> PLGSEEEEEDAGLVAEAEAVAAGWMLDFLCLSLCRAFRDGRSEDFRRTRNSAEAIIHGLSSLTACQLRTIYICQFLTRIAAGKTLDAQFENDERITPLESALMIWGSIEKEHDKLHEEIQNLIKIQAIAVCMENGNFKEAEEVFERIFGDPNSHMPFKSKLLMIISQKDTFHSFFQHFSYNHMMEKIKSYVNYVLSEKSSTFLMKAAAKVVESKR;> SGAVTSFLHSLIIQNEPRFAMFGPGLEELNTSLVLSLMSSEELCPTAGLPQRQIDGIGSGVNFQLNNQHKFNILILYSTTRKERDRAREEHTSAVNKMFSRHNEGDDQQGSRYSVIPQIQKVCEVVDGFI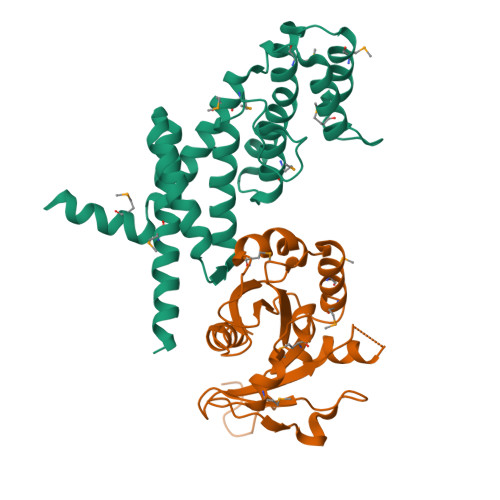YVANAEAHKRHEWQDEFSHIMAMTDPAFGSSGRPLLVLSCISQGDVKRMPCFYLAHELHLNLLNHPWLVQDTEAETLTGFLNGIEWILEEVESKRAR>MAHHHHHHMAKSGLRQDPQSTAAATVLKRAVELDSESRYPQALVCYQEGIDLLLQVLKGTKDNTKRCNLREKISKYMDRAENIKKYLDQEKEDGKYHKQIKIEENATGFSYESLFREYLNETVTEVWIEDPYIRHTHQLYNFLRFCEMLIKRPCKVKTIHLLTSLDEGIEQVQQSRGLQEIEESLRSHGVLLEVQYSSSIHDREIRFNNGWMIKIGRGLDYFKKPQSRFSLGYCDFDLRPCHETT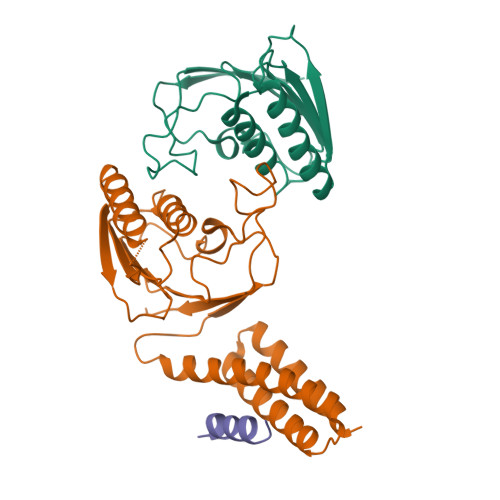VDIFHKKHTKNI[4x];>MEDQLSRRLAALRN[2x]>MSKKQIQPVTRGRAKVPVIMQMEALECGAASLAMVLAYYKKWVPLEQVRVDCGVSRDGSNALNVLKAARNYGLEAKGYRYEPEKLKKEGTFPCIIHWNFNHFVVLKGFKGKYAYINDPAKGDVKIPMEEFDRSFTGICLIFKPTDRF[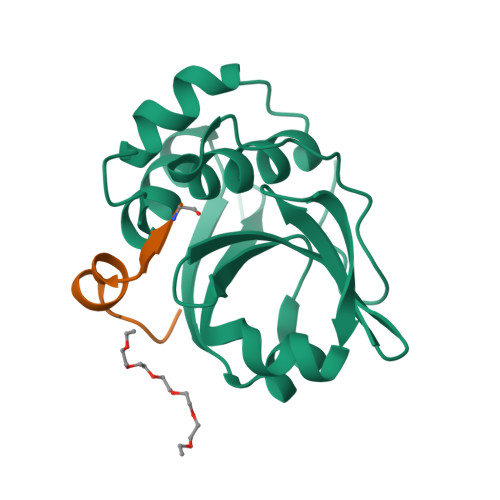4x];>[4x]GNLSDDELEGVAGG> STLKKKRTWHKHGPGQAPDVKPVQNGSQLFIKELRSRTFPSAEDVVARVPGSQLTLGYMEEHGFTEPILVPKKDGLGLAVPAPTFYVSDVENYVGPERSVDVTDVTKQKDCKMKLKEFVDYYYSTNRKRVLNVTNLEFSDTRMSSFVEPPDIVKKLSWVENYWPDDALLAKPKVTKYCL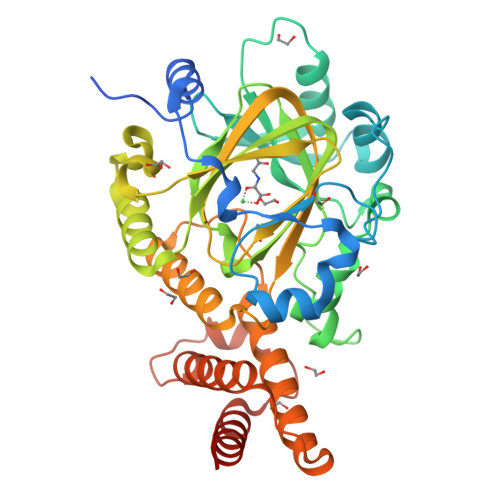ICVKDSYTDFHIDSGGASAWYHVLKGEKTFYLIRPASANISLYERWRSASNHSEMFFADQVDKCYKCIVKQGQTLFIPSGWIYATLTPVDCLAFAGHFLHSLSVEMQMRAYEVERRLKLGSLTQFPNFETACWYMGKHLLEAFKGSHKSGKQLPPHLVQGAKILNGAFRSWTKKQALAEHEDELPEHFKPSQLIKDLAKEIRLSENASKAVRP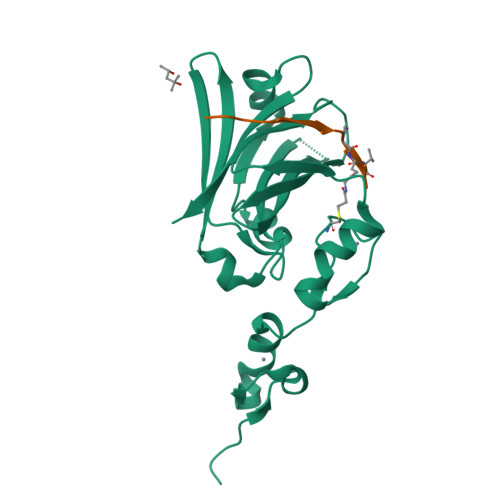>[2x]GSHVANSVLFPCKYASSGCEITLPHTEKADHEELCEFRPYSCPCPGASCKWQGSLDAVMPHLMHQHKSITTLQGEDIVFLATDINLPGAVDWVMMQSCFGFHFMLVLEKQEKYDGHQQFFAIVQLIGTRKQAENFAYRLELNGHRRRLTWEATPRSIHEGIATAIMNSDCLVFDTSIAQLFAENGNLGINVTISMC;>XKLRPVAMVRPXVR[2x]>MLEKEEATTSENSNLVSTDEPHLGGVLAAADVGGKQDATNYNSIFANRFAAFDELLSILKTKFACRVLFEETLVLPKVGRSRLHLCKDGSPRVIKAVGVQRNGSEFVLLEVDVSDGVKMLSTKVLSGVDSETWRNDFEKIRRGVVKSSLNWPNSLFDQLYGQDGHRGVNHPKGLGELQVSRENMEGWAERVVREQFTHLE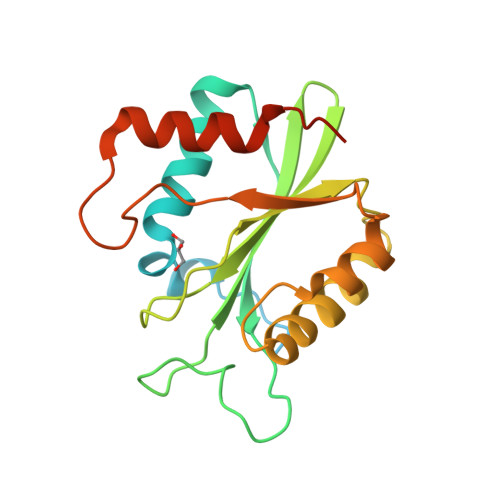HHHHHH[2x]> MMASTSNDEEKLISTTDKYFIEQRNIVLQEINETMNSILNGLNGLNISLESSIAVGREFQSVSDLW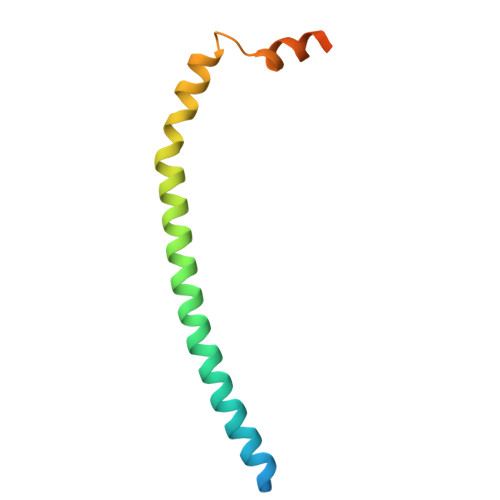KTLYDGLESLSDEAPIDEQPTLSQSKTK>GSFKFTAQQHVYDINGVKVGGQPGEYPTVLIGSIFYRGHKIVSDGQKGIFDKDAAKALLDQEAELSAETGNPFIIDVLGESVEALTKYVEFILENTTAPFLLDSISPDVRVGALKNLGKDPEIQKRLIYNSIEEHYTEEELAAIKEAGLKTAVILAFSKKALKPNARIDLLQGKDDKEGLIAAAKRAGIEQFLVDPGVLDVASNSWTTEAINVVKEQFGYPGGCAPSNAVYLWKKMRSKGTPFFEVAGAAVFTYPITQGADFILYGPMMNAPWVYRAIATTDAMIAYNNKLTGVKMGTTEHPLLKIF[2x]

During energy production in Desulfitobacterium hafniense, MtgA catalyzes the methyl transfer from methylcobalamin (Cbl‐CH3) to THF in the catabolism of glycine betaine (GB). Despite its lack of sequence identity with known structures, we could show that MtgA forms a homodimeric complex of two TIM barrels. The topology of each subunit is characterized by a funnel of eight parallel β‐sheets connected by α‐helices on the outside that form a complex of two perpendicularly oriented TIM barrels. The active‐site cavity is located inside the hydrophilic core of each barrel.

Herein, we present X‐ray structures of THF‐ and THF‐CH3‐bound MtgA that allow us atomic insights into the reaction trajectory of this catalyst. In contrast to substrate‐bound MtgA, the entire cofactor is defined in the MtgA:THF‐CH3 complex depicting extensive coordination within the amino acid environment in a rigid manner. The overall binding motif of the pterin ring remains similar to the substrate‐bound structure. However, the THF benzoate moiety is now involved in a π‐stacking network including Tyr230, Phe243, Phe251, and Trp272 on one side, as well as Tyr35 and His38 on the other. While the functional groups of the THF tail engage water‐coupled hydrogen bonding interactions with adjacent residues, the terminal γ‐carboxylate forms salt bridges with Arg236 that coordinate the cofactor in an extended conformation. Besides this fixation, the superposition of both ligand structures illustrates a rotation of the pterin moiety during the reaction of approximately 35°. In contrast, the benzoate group of THF‐CH3 displaces the carboxamide side chain of Asn227 by 2 Å (red double arrow). As planar sp2 hybridization would be expected in this position of the final product THF‐CH3, the X‐ray structure must depict a trapped protonated reaction intermediate. Notably, the active site lacks residues to deprotonate the (THF‐CH3)+ intermediate; this decreases the conjugated electron system within the pterin ring system. On the other hand, the WT MtgA:THF‐CH3 structure illustrates an intermediate that forms immediately after CH3 transfer from Cbl‐CH3 to THF.>MHIIPVASDPKTCSSGVNENSLDFDFTMAFQPIVNCRTKEIFGY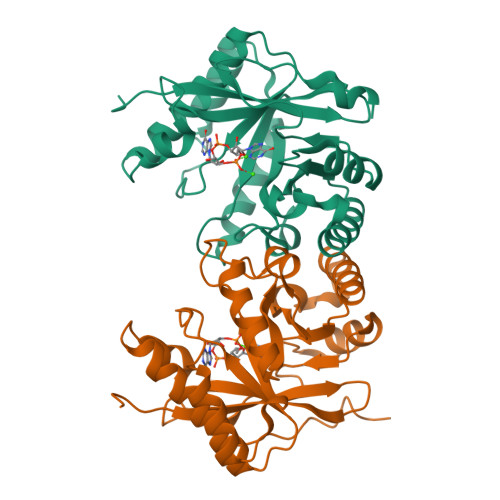EALVRGLNNESAYSVISRVNEDNRYLFDQMCRVKAIALAAKLGLTSKLSINFLPNAIYVPERCIRTTLEAAKRYQFPIENIMFEFTEAERVEDVNHIKRIVEYYKSLGFQTAIDDFGSGYSGLNLLADFQTNIVKVDMGLIRNIHADQVRQSIMKNCLKLFSDLNIQPLAEGVESHAEFAWLKAAGVELMQGYYFAKPGFESLPSVNPEFSEA[4x]>[6x]PRNYERDLQNPDLLVPPITDHGTVSNLRFSFSDAHMRIEEGGWTREVTNRELPASHDLAGVDMCLKPGAYRELHWHKEAEWAFMIAGNARVTALDAEGRSFIDDINAGDLWNFEAGIPHSIQALDQGCEFLLVFSEP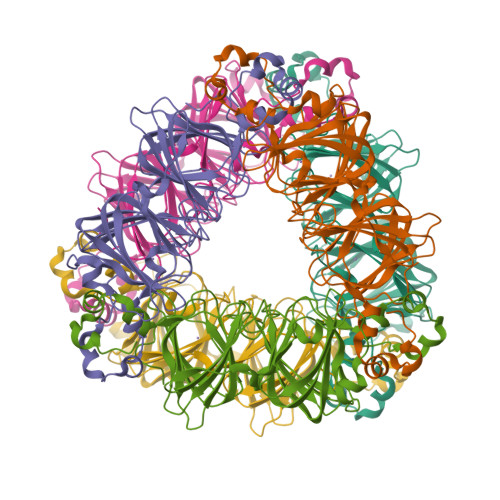DFSENNTFLLTDWLAHTPKDIIAANFKVDESVLANLPGKEKYIFNGEVPGPISEVKKNNPNGDVPSPFTFHMNDLKPHEFEAGKVWIIDSKVFPVAQTISAAIVEIQPGGMRELHWHPKSEEWDYFVQGHAKVGVFNSASLARTFNFQAGDVGVIPIVAGHYIQNIGDEPLIFLEVFKNPIYSDISLNKWLATSPTQMVSDHLNISPETVEQFPKLEHHHHHH> MSGSLQADLGKKSLTRLQAESSAAIHATAKWTTENLAKTQAAQAERAKAAMLSQQAAKAKQAKLTQHLKDVVDRALQNNKTRPTVIDLAHQNNQQMAAMAEFIGRQKAIEEARKKAEREAKRAEEAYQAALRAQEEEQRKQAEIERKLQEARKQEAAAKAKAEADRIAAEKAEAEARAKAEAERRKAEEARKALFAKAGIKDTPLEHHHHHH

Here, we use biochemical, biophysical and structural analyses to show how a bacteriocin exploits TolC, a major outer-membrane antibiotic efflux channel in Gram-negative bacteria, to transport itself across the outer membrane of target cells. Klebicin C (KlebC), a rRNase toxin produced by Klebsiella pneumoniae, binds TolC of a related species (K. quasipneumoniae) with high affinity through an N-terminal, elongated helical hairpin domain common amongst bacteriocins. TolC is one of the most prevalent drug efflux channels in bacteria and is frequently associated with multidrug resistance. Our results indicate that TolC, in addition to its known role in antibiotic export, can function as a protein import channel for bacteriocins.

Crystallisation screens were focused solely on KlebC51-254 since this construct retained TolC-binding activity (similar to KlebC1-271) whilst removing the putative disordered region at the N-terminus. Crystals of selenomethionine-labelled KlebC51-254 were obtained in the P3221 space group. The resulting structure, solved by single-wavelength anomalous diffraction to a resolution of 1.9 Å, revealed a helical hairpin spanning 150 Å. Modelled density spanned Lys62 to Leu255, with residues 64–131 forming helix 1 of the hairpin and helix 2 containing residues 145–248. The lack of density for residues 51–61 suggest that the disorder predicted for the first 50 residues may extend further into the molecule. We explored this possibility with heteronuclear NMR experiments and found that indeed the first 60 residues of KlebC are disordered in solution. In the crystal structure of the KlebC51-254 isolated helical hairpin, residues Asp137 to Gln144 comprise the linker sequence between helix 1 and helix 2. Using disulphide-by-design, two interhelical disulphide bonds were engineered (L86C, L198C and A107C, Y177C) to lock the helical hairpin in the conformation observed in the crystal structure. In their reduced forms, both L86C, L198C KlebC1-254 and A107C, Y177C KlebC1-254 bound TolC, but in their oxidised states neither protein could bind TolC. These experiments indicate that TolC binding requires the helical hairpin to undergo a gross conformational change from that observed in the crystal structure.> GSHMKDLRSPICCILGHVDTGKTKLLDKIRQTNVQGGEAGGITQQIGATYFPIDAIKAKTKVMAEYEKQTFDVPGLLVIDTPGHESFSNLRSRGSSLCNIAILVIDIMHGLEQQTIESIKLLRDRKAPFVVALNKIDRLYDWKAIPNNSFRDSFAKQSRAVQEEFQSRYSKIQLELAEQGLNSELYFQNKNMSKYVSIVPTSAVTGEGVPDLLWLLLELTQKRMSKQLMYLSHVEATILEVKVVEGFGTTIDVILSNGYLREGDRIVLCGMNGPIVTNIRALLTPQPLRELRLKSEYVHHKEVKAALGVKIAANDLEKAVSGSRLLVVGPEDDEDELMDDVMDDLTGLLDSVDTTGKGVVVQASTLGSLEALLDFLKDMKIPVMSIGLGPVYKRDVMKASTMLEKAPEYAVMLCFDVKVDKEAEQYAEQEGIKIFNADVIYHLFDSFTAYQEKLLEERRKDFLDYAIFPCVLQTLQIINKR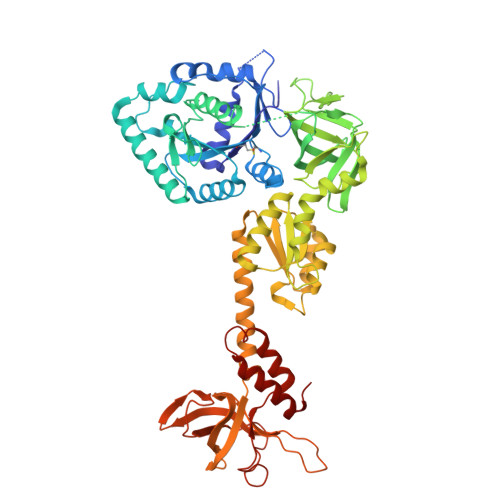GPMIIGVDVLEGTLRVGTPICAVKTDPTTKERQTLILGKVISLEINHQPVQEVKKGQTAAGVAVRLEDPSGQQPIWGRHVDENDTLYSLVSRRSIDTLKDKAFRDQVARSDWLLLKKLKVVFGIE> SMPKTISVRVTTMDAELEFAIQPNTTGKQLFDQVVKTIGLREVWFFGLQYQDTKGFSTWLKLNKKVTAQDVRKESPLLFKFRAKFYPEDVSEELIQDITQRLFFLQVKEGILN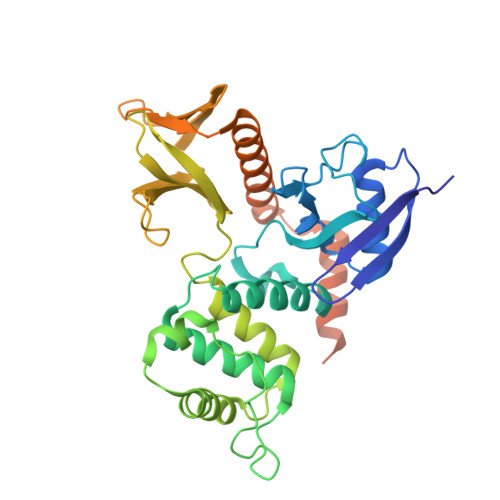DDIYCPPETAVLLASYAVQSKYGDFNKEVHKSGYLAGDKLLPQRVLEQHKLNKDQWEERIQVWHEEHRGMLREDAVLEYLKIAQDLEMYGVNYFSIKNKKGSELWLGVDALGLNIYEQNDRLTPKIGFPWSEIRNISFNDKKFVIKPIDKKAPDFVFYAPRLRINKRILALCMGNHELYMRRRKPDTIEVQQMKAQAREEKHQKQMERAMLENEKKKREMAEKEKEKIEREKEE>[6x]XGELKAIAQEL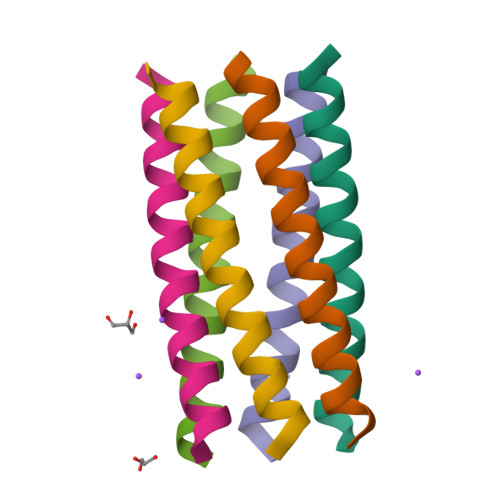KAIAKELKAIAWEDKAIAQGAGYX> GSGLGLTPEQKQKKAALSASEGEEVPQDKAPSHVPFLLIGGGTAAFAAARSIRARDPGARVLIVSEDPELPYMRPPLSKELWFSDDPNVTKTLRFKQWNGKERSIYFQPPSFYVSAQDLPHIENGGVAVLTGKKVVQLDVRDNMVKLNDGSQITYEKCLIATGGTPRSLSAIDRAGAEVKSRTTLFRKIGDFRSLEKISREVKSITIIGGGFLGSELACALGRKARALGTEVIQLFPEKGNMGKILPEYLSNWTMEKVRREGVKVMPNAIVQSVGVSSGKLLIKLKDGRKVETDHIVAAVGLEPNVELAKTGGLEIDSDFGGFRVNAELQARSNIWVAGDAACFYDIKLGRRRVEHHDHAVVSGRLAGENMTGAAKPYWHQSMFWSDLGPDVGYEAIGLVDSSLPTVGVFAKATAQDNPKSATEQSGTGIRSESETESEASEITIPPSTPAVP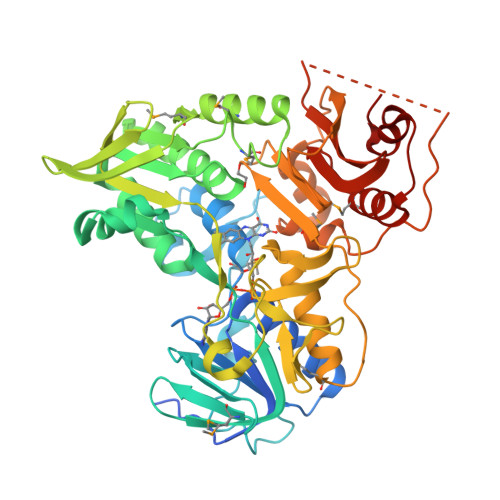QAPVQGEDYGKGVIFYLRDKVVVGIVLWNIFNRMPIARKIIKDGEQHEDLNEVAKLFNIH>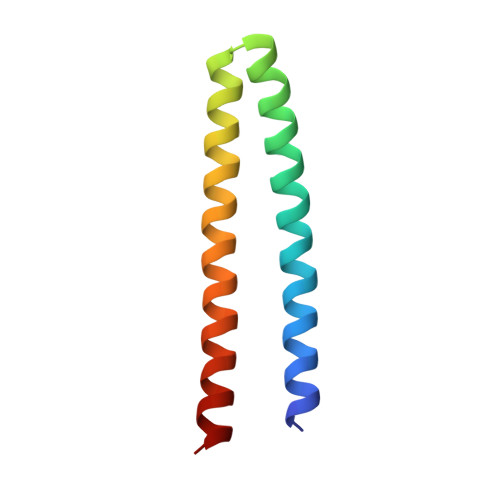 GSKQKEAIKVYLELLEVHSRVLKALIEQIKLFIELIKRPDEDLADKVRKSSEELKKIIKEVEKILRKVDDILYKVKS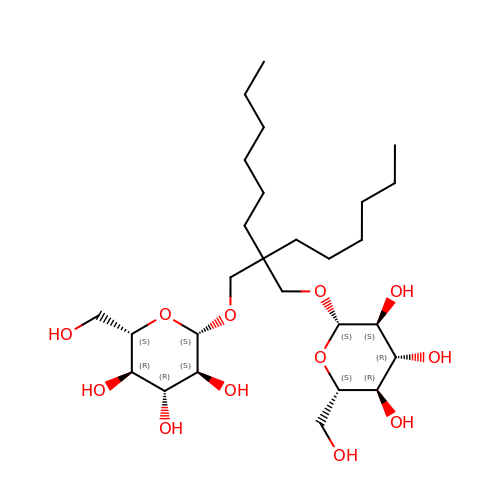Octyl Glucose Neopentyl Glycol  | C27 H52 O12 | TYXCLOLHZMMLEK-RNDJEAJNSA-N4-azanyl-1-[(2~{R},3~{R},4~{S},5~{R})-5-(hydroxymethyl)-3,4-bis(oxidanyl)thiolan-2-yl]pyrimidin-2-one | C9 H13 N3 O4 S | 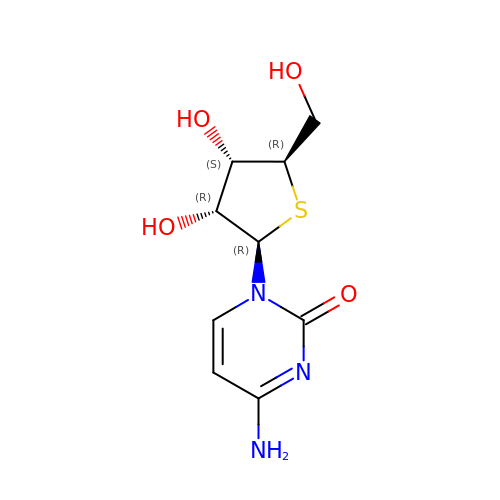GAKJJSAXUFZQTL-XVFCMESISA-N>[4x]ADKELKFLVVDDFSTMRRIVRNLLKELGFNNVEEAEDGVDALNKLQAGGYGFVISDWNMPNMDGLELLKTIRADGAMSALPVLMVTAEAKKENIIAAAQAGASGYVVKPFTAATLEEKLNKIFEKLGM;>[4x]RQLALEAKGETPSAVTRLSVVAKSEPQDEQSRSQSPRRIILSRLKA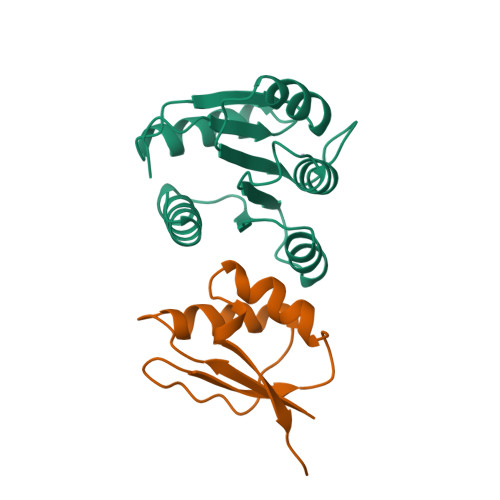GEVDLLEEELGHLTTLTDVVKGADSLSAILPGDIAEDDITAVLCFVIEADQITFETVEVSPKISTPPVLKLAAEQAPTGRVEREKTTR>GEDVFEVEKILDMKTEGGKVLYKVRWKGYTSDDDTWEPEIHLEDCKEVLLEFRKKIAENKAK[2x]

M-phase phosphoprotein 8 (MPP8) was initially identified to be a component of the RanBPM-containing large protein complex, and has recently been shown to bind to methylated H3K9 both in vivo and in vitro. MPP8 binding to methylated H3K9 is suggested to recruit the H3K9 methyltransferases GLP and ESET, and DNA methyltransferase 3A to the promoter of the E-cadherin gene, mediating the E-cadherin gene silencing and promote tumor cell motility and invasion. MPP8 contains a chromodomain in its N-terminus, which is used to bind the methylated H3K9. Here, we reported the crystal structures of human MPP8 (hMPP8) chromodomain both in free form and in complex with the trimethylated histone H3 lysine 9 (H3K9me3) peptide (residue 1–15).

To unveil the molecular architecture of the chromodomain of hMPP8, hMPP8 chromodomain (55–116 residues) was recombinantly expressed and crystallized. In the free form, the hMPP8 chromodomain consists of a twisted anti-parallel β-sheet formed by three β-strands (named β2–β4), and α helix (named αA) located at the C-terminal end packing against one edge of the β-sheet next to β2. In the asymmetric unit of the crystal, two hMPP8 chromodomain monomers form a dimer through the interaction between the β2 strand from each monomer. The β2 strand from one subunit runs anti-parallel to the β2' strand from the neighboring one, pulling the three-stranded anti-parallel β-sheets of two hMPP8 chromodomain proteins adjacent to constitute a six-stranded anti-parallel β-sheet. Specifically, Asp66, Met67, Thr69, Gly71 and Gly72 of β2 strand form hydrogen bond with Gly72', Gly71', Thr69', Met67' and Asp66' of β2' strand from the opposite subunit, respectively. The dimer interface has a buried surface area of about 1025 Å2, which is strong enough to form a stable dimer. Sequence alignment result indicates that hMPP8 chromodomain is more similar to HP1 choromodomain and lacks the residues in dPlycomb chromodomain for dimerization. It was quite unexpectedly to find that hMPP8 chromodomain forms homodimer in our crystal structures. To determine the oligomerization state of hMPP8 chromodomain in solution, size exclusion experiment was performed. The size of hMPP8 chromodomain in solution is corresponding to dimer, consistent with the observation in crystal structure. Therefore, the chromodomain exists as a homodimer in solution and the homodimer structure in crystal is not due to crystal packing.Lysine lactylation (Kla) is a novel histone post-translational modification discovered in late 2019. Emerging biological and structural evidence suggests that Sirtuins are not limited to erasing acetyl groups from lysine residues but can also remove other forms of acyl groups. The zinc-binding domain and Rossmann fold domain make up the highly conserved catalytic core of Sirtuins. Our findings indicate that SIRT3 exhibits higher delactylation activity compared to other human Sirtuins, especially on H4K16 site.

Crystals of H3K23la(L)-SIRT3 and H4K16la(L)-SIRT3 complexes diffracted to 2.0 Å and 2.5 Å resolution, respectively. Each structure contains 1 SIRT3 molecule, 1 zinc atom, and 1 lactyl peptide in each asymmetric unit. The catalytic pocket of SIRT3 displayed half-hydrophobic and half-hydrophilic characters. In both structures, F180, I230, I291, and V292 of SIRT3 formed a preconfigured hydrophobic cage that accommodated the hydrocarbon portion of the lactyl group. Several water molecules participated in the hydrogen bond network to facilitate the interaction between the hydroxyl group of the Kla and Q228, N229, H248 of SIRT3 in SIRT3-H4K16la(L) structure. Furthermore, a water bridge network involving Q228, N229, and H248 of SIRT3 stabilizes the hydroxyl group of lactyl-lysine. The fitted curve calculated KM = 142.66 ± 2.64 μM, Vmax = 0.925 ± 0.101 μmol/L/min, kcat = 0.08 ± 0.008 s−1, kcat/KM = 5.40∗102 s−1M−1. Knocking down either SIRT3 or HDAC3 increased cellular H4K16la level. The binding affinity of SIRT3 to lactylated D-lysine peptide was also found to be approximately 2-fold higher than that of lactylated L-lysine peptide. Hence, the probe p-H4K16laAlk validated that H4K16la is the substrate of SIRT3 in cellualr environment.

> DKGKLSLQDVAELIRARACQRVVVMVGAGISTPSGIPDFRSPGSGLYSNLQQYDLPYPEAIFELPFFFHNPKPFFTLAKELYPGNYKPNVTHYFLRLLHDKGLLLRLYTQNIDGLERVSGIPASKLVEAHGTFASATCTVCQRPFPGEDIRADVMADRVPRCPVCTGVVKPDIVFFGEPLPQRFLLHVVDFPMADLLLILGTSLEVEPFASLTEAVRSSVPRLLINRDLVGPLAWHPRSRDVAQLGDVVHGVESLVELLGWTEEMRDLVQRETGKLDGPDK;> GGAKRHRK>MGKGIIVRVPHGIELSSELLSALEVRFPGYILETYYQKPDYHRSFARRVDSLHKAFYFLIDAYPFSAKNTPLTKQTLKAYVDECKLATTDAKGSIDDLHKELERFTAKLIELIAL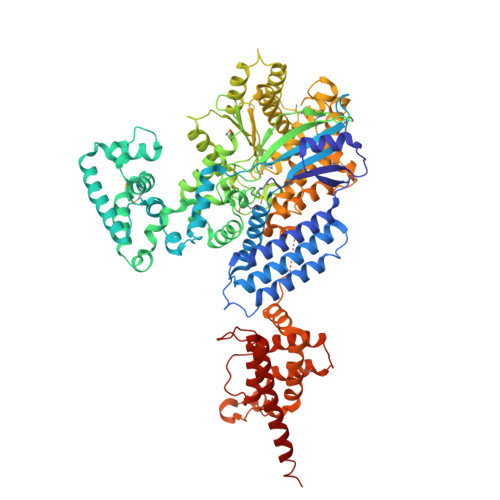NWGCSEIKEAVELLNEAEQYALMGEGRYDLVTLLPMQLGQDVDYVLQVDESLPPYYDQLLDELTLIKAKKYPKTPGWLRDLEEYQHAYFCNLDQGVTSYLEVIRDFNNFLLNWASIKKIALSLNSDLQQIVSGSPPLPSWFNGLSVHQREMMRILAADPTSLDKKLTQFKKFLTGDIKWEIWDTATQISSLPQWYWVLSEHQQFFLEHVLKGVDDVKDAVSFLSSRHRTLPLPANYAAHSLLGLSENGNMRELSAKRYRSSHIATRDGLNWPKAVQQRHSDSNLAKVMEYSKNDQLAILQTLISPIHATEYVPNWITDYLPTLPPDLDLYKLARSAVERRKETQSILQNNHPYNMAKRLYYTQAYDKDSQSLLVTAKKYASFTPGLQELLDQYQSVLESALGTATIFDYAGRELFLSSLEQLIILTIGGHSYGSCVSGKDRKAIELIHTDAMILYKECYGTWPVFDELPDKENRIRFVSLVADLYMSRHQHEHAGQNAPGSEGIKTPEWYLPEDIAAEIRKRLDSERSLKDDDRAATDNEVKNIFIGGSKKLKEYLLPEKKLLCRLVARQLGESNCTKLYDALHSLINERNLFTPQEQSSRWTSSFFSSESNPTPDGIKQILELMLSPSSGKDNIIRIEKILQVVSERPEIDGSRTEATNSVYGRLRSFLNCSEKATTFSEIVSTTVEEWTKLFEESKRAHVKEFESSHR[2x]>HFLCGVVEGFYGRPWVMEQRKELFRRLQKWELNTYLYAPKDDYKHRMFWREMYSVEEAEQLMTLISAAREYEIEFIYAISPGLDITFSNPKEVSTLKRKLDQVSQFGCRSFALLFDNIDHNMCAADKEVFSSFAHAQVSITNEIYQYLGEPETFLFCPTEYCGTFCYPNVSQSPYLRTVGEKLLPGIEVLWTGPKVVSKEIPVESIEEVSKIIKRAPVIWDNIHANDYDQKRLFLGPYKGRSTELIPRLKGVLTNPNCEFEANYVAIHTLATWYKSNMNGVRKDVVMTDSEDSTVSIQIKLENEGSDEDIETDVLYSPQMALKLALTEWLQEFGVPHQYSSRGGGGSGGGGSVTLEDLQ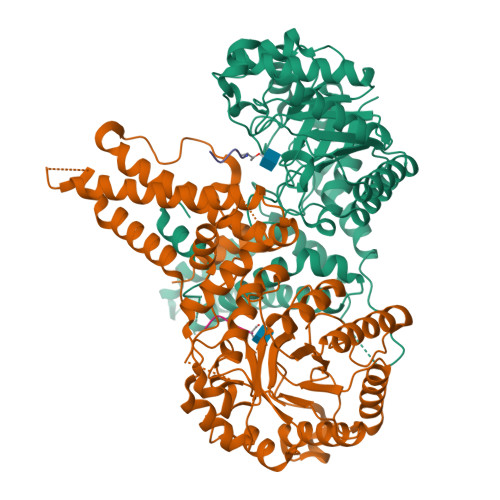LLADLFYLPYEHGPKGAQMLREFQWLRANSSVVSVNCKGKDSEKIEEWRSRAAKFEEMCGLVMGMFTRLSNCANRTILYDMYSYVWDIKSIMSMVKSFVQWLGCRSHSSAQFLIGDQEPWAFRGGLAGEFQRLLPIDGANDLFFQ[2x];>KLSPSPSSRVTVS[2x]>[12x]MRVIFSEDHKLRNAKTELYGGELVPPFEAPFRAEWILAAVKEAGFDDVVAPARHGLETVLKVHDAGYLNFLETAWDRWKAAGYKGEAIATSFPVRRT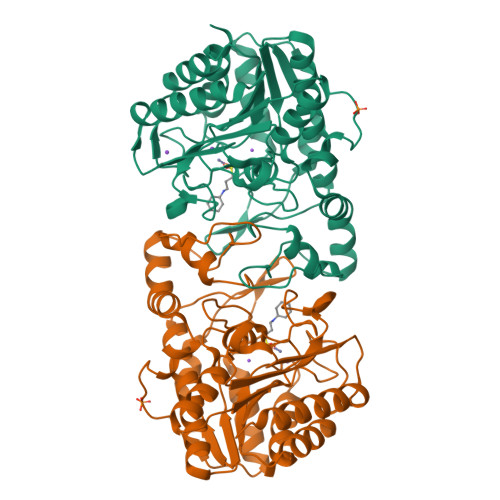SPRIPTDIEGQIGYYCNAAETAISPGTWEAALSSMASAIDGADLIAAGHKAAFSLCRPPGHHAGIDMFGGYCFINNAAVAAQRLLDKGAKKIAILDVDFHHGNGTQDIFYERGDVFFASLHGDPAEAFPHFLGYAEETGKGAGAGTTANYPMGRGTPYSVWGEALTDSLKRIAAFGAEAIVVSLGVDTFEQDPISFFKLTSPDYITMGRTIAASGVPLLVVMEGGYGVPEIGLNVANVLKGVAG(2R)-2-hydroxy-3-(morpholin-4-yl)propane-1-sulfonic acid | C7 H15 N O5 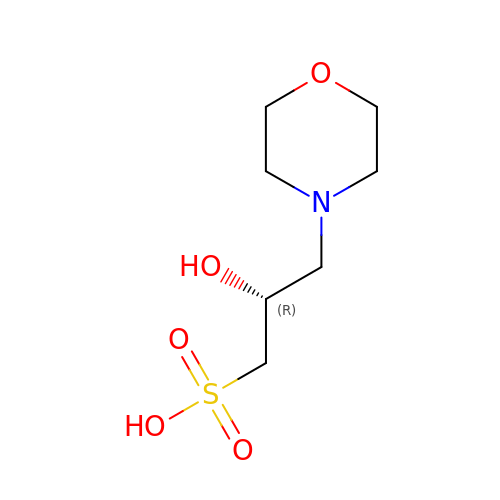S | NUFBIAUZAMHTSP-SSDOTTSWSA-N'5'-O-(N-(L-ALANYL)-SULFAMOYL)ADENOSINE | C13 H19 N7 O7 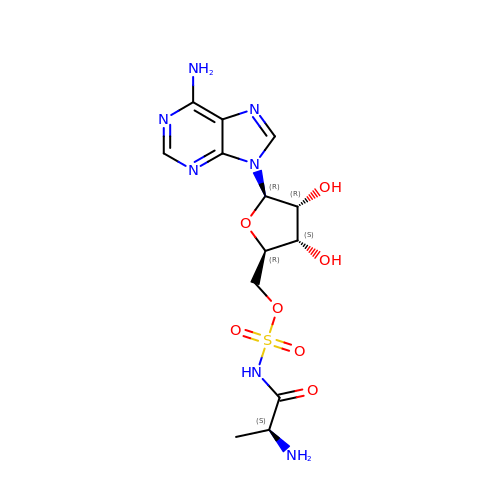S | CWWYMWDIYBJVLP-YTMOPEAISA-N> GPMFEARLVQGSILKKVLEALKDLINEACWDISSSGVNLQSMDSSHVSLVQLTLRSEGFDTYRCDRNLAMGVNLTSMSKILKCAGNEDIITLRAEDNADTLALVFEAPNQEKVSDYEMKLMDLDVEQLGIPEQEYSCVVKMPSGEFARICR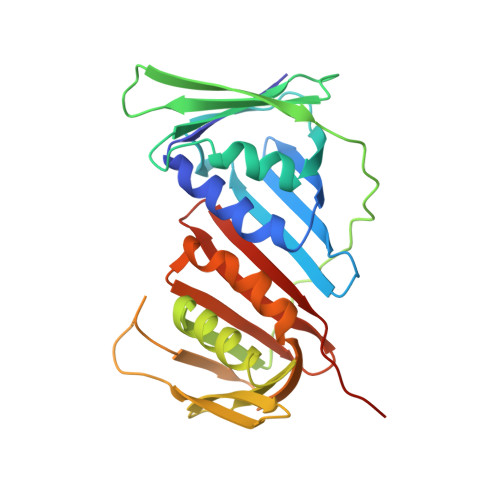DLSHIGDAVVISCAKDGVKFSASGELGNGNIKLSQTSNVDKEEEAVTIEMNEPVQLTFALRYLNFFTKATPLSSTVTLSMSADVPLVVEYKIADMGHLKYYLAPKIEDEEGS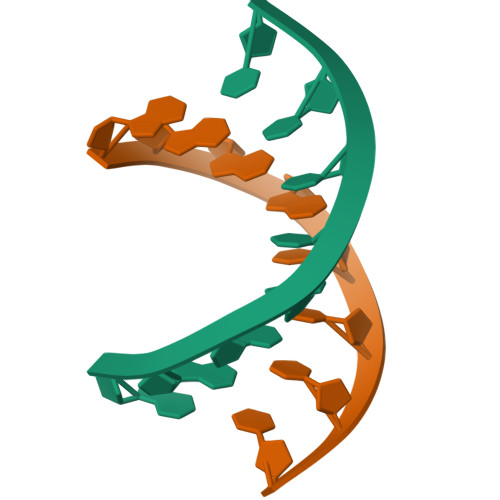>GGGGTCCC[2x]Aurora A, a Ser/Thr kinase, is a key regulator of mitotic events, including mitotic entry, centrosome maturation, and spindle formation. Aurora A depletion leads to cell cycle arrest, while overexpression has been found in many cancer cell lines. TPX2 recruits Aurora A to the spindle microtubules, an event that is essential in spindle formation. Here we investigate two fundamentally distinct regulation mechanisms by characterizing autophosphorylation of Aurora A as well as activation by TPX2 (Targeting Protein for Xklp2).

We first solved the crystal structure of dephosphorylated Aurora A in the absence and presence of TPX21−45 and bound to an ATP-mimic (β,γ-methyleneadenosine 5′ triphosphate, AMPPCP). Comparison of dephosphorylated Aurora A in the absence or presence of TPX2 reveals subtle but significant interactions by which TPX2 stabilizes the active form of the kinase. First, binding of TPX2 causes a slight rotation of the αC-helix towards the catalytic center, thus allowing for the conserved, stabilizing E181-K162 ion pair to form. The αC-helix rotation also results in movement of F275 of the conserved DFG motif from the DFG-out into the DFG-in position (bottom inset). Second, movement of F275 initiates a cascade of side chain interactions that result in the completion of the regulatory spine originating from the αF-helix (R-spine). From these structural features it appears that Aurora A, despite being dephosphorylated, is in an active conformation when bound to TPX2. Curiously, the last two hallmarks of the active state are created by a swap of the activation segments of Aurora A resulting in a dimer conformation that has not been previously reported for this protein. In contrast we find an asymmetric dimer within the unit cell with monomer I showing complete electron density for the activation segment while monomer II is missing residues 283–288 (red and blue, respectively). In addition, only monomer I has the perfect geometry of the conserved hydrogen bond network found in a catalytically prone kinase between residues D256, K258, and T292. Therefore we speculated that monomer I may be the enzyme molecule recognizing monomer II as its substrate.

>[2x]ESKKRQWALEDFEIGRPLGKGKFGNVYLAREKQSKFILALKVLFKAQLEKAGVEHQLRREVEIQSHLRHPNILRLYGYFHDATRVYLILEYAPLGTVYRELQKLSKFDEQRTATYITELANALSYCHSKRVIHRDIKPENLLLGSAGELKIADFGWSVHAPSSRRTTLCGTLDYLPPEMIEGRMHDEKVDLWSLGVLCYEFLVGKPPFEANTYQETYKRISRVEFTFPDFVTEGARDLISRLLKHNPSQRPMLREVLEHPWITANSSKPSNCQNKESASKQS;>[2x]MSQVKSSYSYDAPSDFINFSSLDDEGDTQNIDSWFEEKANLEN>[4x]MGQGDESERIVINVGGTRHQTYRSTLRTLPGTRLAWLAEPDAHSHFDYDPRADEFFFDRHPGVFAHILNYYRTGKLHCPADVCGPLYEEELAFWGIDETDVEPCCWMTYRQHRDAEEALDSFGGAPLDNSADDADADGPGDSGDGEDELEMTKRLALSDSPDGRPGGFWRRWQPRIWALFEDPYSSRYARYVAFASLFFILVSITTFCLETHERFNPIVNKTEIENVRNGTQVRYYREAETEAFLTYIEGVCVVWFTFEFLMRVIFCPNKVEFIKNSLNIIDFVAILPFYLEVGLSGLSSKAAKDVLGFLRVVRFVRILRIFKLTRHFVGLRVLGHTLRASTNEFLLLIIFLALGVLIFATMIYYAERIGAQPNDPSASEHTHFKNIPIGFWWAVVTMTTLGYGDMYPQTWSGMLVGALCALAGVLTIAMPVPVIVNNFGMYYSLAMAKQKLPKKKKKHIPRPPQLGSPNYCKSVVNSPHHSTQSDTCPLAQEEILEINRAGRKPLRGMSIGSLEVLFQ

Voltage-gated potassium channels (Kv) form a family of transmembrane ion channels which are voltage-sensitive and selective for potassium ions. Kv3.1 channels conduct a delayed rectifying outward current and have a high activation threshold (≈ −20 mV) as well as rapid activation and deactivation kinetics. The Kv3.1 channels are, thereby responsible for neuronal repolarization, and high-frequency action potential firing. The Kv3 channels, like other Kv channels, are tetrameric structures of four pore-forming alpha subunits.

The cryo-EM structure of flWT-Kv3.1a was solved at 2.65 Å overall resolution. Human flWT-Kv3.1a adopts a tetrameric swapped organization, with the VSD of each subunit interacting with the PD of the neighboring subunit. In contrast, the T1 cytoplasmic domain shows a novel structural feature by adopting a 35° twisted conformation. Another major dissimilarity is the zinc-binding site at the base of the T1 tetramerization, which is not observed in Kv1.2. The structure of flWT-Kv3.1a shows that only Arginines R1, R2, and R3 are located above the Phe256 residue within the hydrophobic charge transfer center, which in general consists of a rigid cyclic cap and two negatively charged residues interacting with a positively charged residue in S4, and which facilitates the movement of positively charged residues through the membrane. Arginine R4, which is located above the residue Phe233 (equivalent to Phe256 in Kv3.1) in the structure of Kv1.2–Kv2.1, is in the case of Kv3.1 involved in a Π–cation interaction with Phe256. Overall the S4 sensor of Kv3.1, which is characterized by high activation potential, is shifted downward, in comparison to the structure of Kv1.2–Kv2.1. A total of four sites of potassium ions could be modeled coordinating the residues forming the selectivity filter. The analysis of the pore radius in this region shows that the lower gate of the channel is in an open conformation with a diameter of 3.3 Å, similar to other structures solved in the open state, such as Kv1.2 (4, 20–22) and Kv7.1 (25, 26) with similar pore radius at the most constricted region.> MASEFKKKLFWRAVVAEFLATTLFVFISIGSALGFKYPVGNNQTAVQDNVKVSLAFGLSIATLAQSVGHISGAHLNPAVTLGLLLSCQISIFRALMYIIAQCVGAIVATAILSGITSSLTGNSLGRNDLADGVNSGQGLGIEIIGTLQLVLCVLATTDRR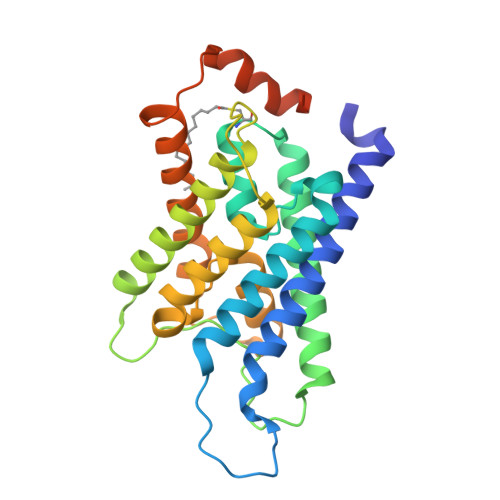RRDLGGSAPLAIGLSVALGHLLAIDYTGCGINPARSFGSAVITHNFSNHWIFWVGPFIGGALAVLIYDFILAPRSSDLTDRVKVWTSGQVEEYDLDADDINSRVEMKPK>TDLKASSLRALKLMHLATSANDDDTDEKVIALCHQAKTPVGTTDAIFIYPRFIPIARKTLKEQGTPEIRICTSTNFPHGNDDIDIALAETRAAIAYGADSVAVVFPYRALMAGNEQVGFDLVKACKEACAAANVLLAVIIETGELKDEALIRKASEISIKAGADNIVTSTGKVAVGATPESARIMMEVIRDMGVEKTVGFIPVGGVRTAEDAQKYLAIADELFGADWADARHYAFGASASLLASLL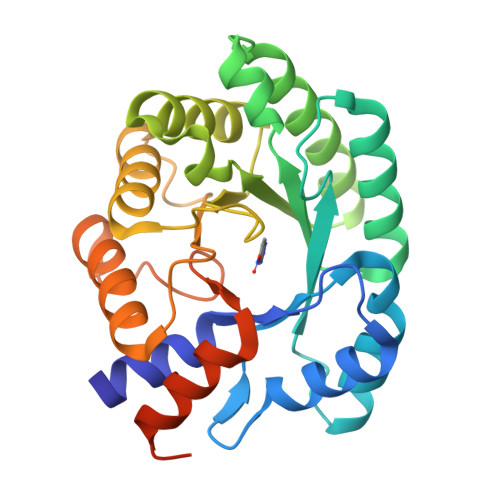KALGHGDGKSASSYGSLEHHHHHH[6x]>[3x]FSSREQPQQNECQIQKLNALKPDNRIESEGGLIETWNPNNKPFQCAGVALSRCTLNRNALRRPSYTNGPQEIYIQQGKGIFGMIYPGSPSTFEEPQQPQQRGQSSRPQDRHQKIYNFREGDLIAVPTGVAWWMYNNEDTPVVAVSIIDTNSLENQLDQMPRRFYLAGNQEQEFLKYQQEQGGHQSQKGKHQQEEENEGGSILSGFTLEFLEHAFSVDK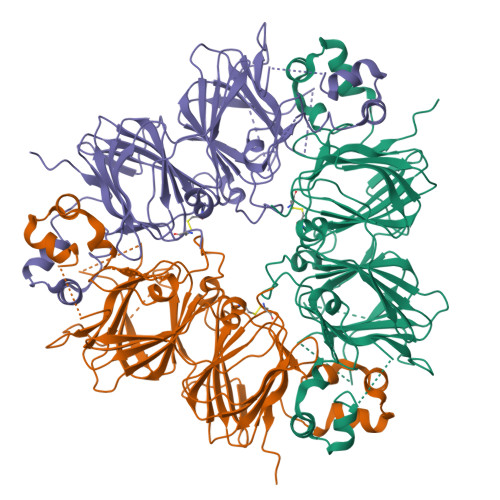QIAKNLQGENEGEDKGAIVTVKGGLSVIKPPTDEQQQRPQEEEEEEEDEKPQCKGKDKHCQRPRGSQSKSRRNGIDETICTMRLRHNIGQTSSPDIYNPQAGSVTTATSLDFPALSWLRLSAEFGSLRKNAMFVPHYNLNANSIIYALNGRALIQVVNCNGERVFDGELQEGRVLIVPQNFVVAARSQSDNFEYVSFKTNDTPMIGTLAGANSLLNALPEEVIQHTFNLKSQQARQIKNNNPFKFLVPPQESQKRAVA>MKTIFSAICPTGVITIGRYIGALRQFVELQHEYNCYFCIADQSAITVWQDPHELRQNIRRLAALYLAVGIDPTQATLFIASEVPAHAQAAWMLQCIVYIGELERMTLFKELSAGKEAVSAGLLTHPPIYAAMILLYNTDIVPVGEYGKQLYELTRDLAERFNKRYGELFTIPEARIPKVGARIMSLVDPTKSMYQSDPNPKAYITLLDDAKTIEKKIKSAVTDSEGTIRYDKEAKPGISNLLNIYSTLSGQSIEELERQYEGKGYGVFKADLAQVVIETLRPIQER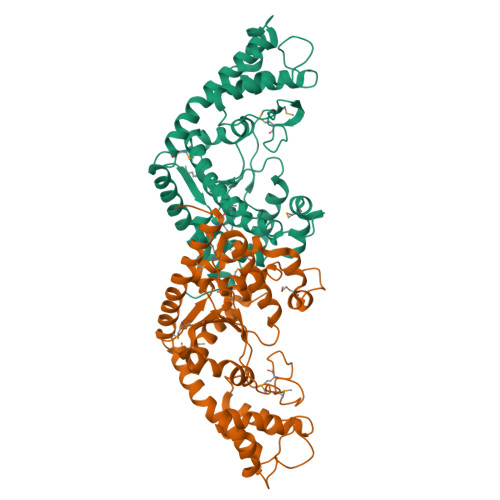YHHWMESEELDRVLDEGAEKANRVASEMVRKMEQAMGLGRRRGSLEHHHHHH[4x]>GSHMALALVGEKIDRNRFTGEKIENSTFFNCDFSGADLSGTEFIGCQFYDRESQKGCNFSRAMLKDAIFKSCDLSMADFRNSSALGIEIRHCRAQGADFRGASFMNMITTRTWFCSAYITNTNLSYANFSKVVLEKCELWENRWIGAQVLGATFSGSDLSGGEFSTFDWEAANFTHCDLTNSELGDLDIRGVDLQGVKLDNYQASLLMERLGIAVIG[2x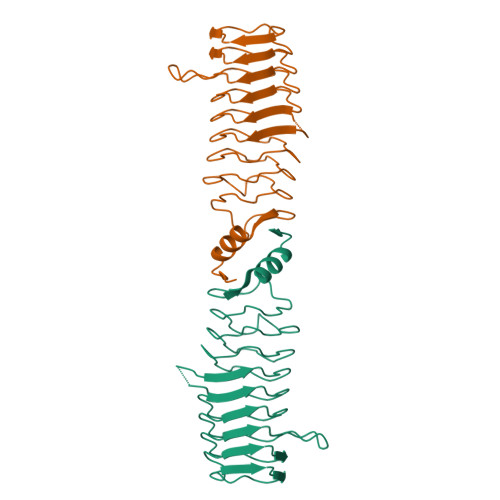]> MHHHHHHSSGMSWTVDIPKEVLPDLPPLPEGMQQQFEDTISRDAKQQPTWDRAQAENVRKILESVPPIVVAPEVLELKQKLADVANGKAFLLQGGDCAETFESNTEPHIRANVKTLLQMAVVLTYGASTPVIKMARIAGQYAKPRSSDLDGNGLPNYRGDIVNGVEATPEARRHDPARMIRAYANASAAMNLVRALTSSGTADLYRL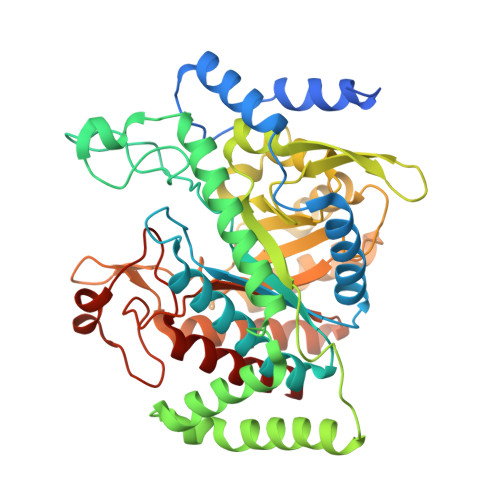SEWNREFVANSPAGARYEALAREIDSGLRFMEACGVSDESLRAADIYCSHEALLVDYERSMLRLATDEEGNEELYDLSAHQLWIGERTRGMDDFHVNFASMISNPIGIKIGPGITPEEAVAYADKLDPNFEPGRLTIVARMGHDKVRSVLPGVIQAVEASGHKVIWQSDPMHGNTFTASNGYKTRHFDKVIDEVQGFFEVHRALGTHPGGIHIEFTGEDVTECLGGAEDITDVDLPGRYESACDPRLNTQQSLELAFLVAEMLRN6-[(~{S})-oxidanyl(phosphono)methyl]pyridine-2-carboxylic acid | C7 H8 N O6 P | 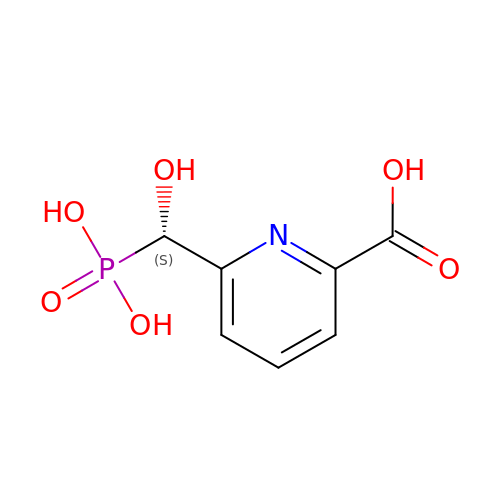BMLFSBIYIPWZDN-ZETCQYMHSA-N> MACPISQSVSQPVDERLTRAAIFLVVTINPGKAAEVAVRTLCGTLSSLVRGVGFRILDGGLSCVMGVSSGGWERLFGDEKPEYLHVFQEINGVHHAPSTPGDLLFHIRAARMDLCFELASRILSDLGSSVCVVDSVQGFRYFDDRDLLGFVDGTENPVAQAAVDATLIGEEDHTFSGGSYVIVQKYLHDLDKWNAIPVEQQEKIIGREKLSDIELKDADKPSYAHNVLTSIEEDGEDVDILRDNMPFGDPGKGEFGTYFIGYSRKPARIERMLENMFVGNPPGNYDRILDVSRAITGTLFFIPTVSFLDSVEPQPSVSQQTDDAKYIYDSPGTKGESGSLNIGSLKKEVQDEENLYFQGGSGGHHHHHHH

Encapsulins are self-assembling protein nanocompartments capable of selectively encapsulating dedicated cargo proteins, including enzymes involved in iron storage, sulfur metabolism, and stress resistance. Encapsulation is mediated by specific cargo protein motifs known as targeting peptides (TPs), though the structural basis for encapsulation of the largest encapsulin cargo class, dye-decolorizing peroxidases (DyPs), is currently unknown. In this study, we report the structural and functional analysis of a DyP encapsulin system from a Gram-negative pathogen – Klebsiella pneumoniae (Kp). DyPs are ubiquitous, often homohexameric, heme-containing enzymes, named for their ability to oxidize and degrade a wide range of synthetic dyes – with concomitant reduction of hydrogen peroxide to water.

To investigate the influence of encapsulation on KpDyP and to compare the activities of encapsulated and free enzyme, a C-terminally His-tagged KpDyP construct (40.6 kDa) was heterologously expressed and purified. The structure of the free KpDyP hexamer was determined to 2.4 Å via D3 symmetry refinement followed by local refinement. The overall structure corroborates our biophysical and imaging analyses and confirms that free KpDyP exists as a catalytically competent hexamer. Cryo-EM density for a non-covalently bound heme cofactor – one per subunit – is clearly visible. The heme group is coordinated by residue His225, representing the proximal ligand to the heme iron. Arg242 is the residue closest to the heme iron on the distal face of the heme group. Moreover, the heme cofactor is substantially buried, with the entrance to the active site partially obstructed by an adjacent subunit at the two-fold interface. The KpDyP surface was found to be predominantly negatively charged, which is in agreement with its theoretical isoelectric point (pI) of 4.6552. The entrance to the active site is also highly negatively charged. In line with the predicted disordered state of the C-terminus, the last 60 residues – including the TP – are unresolved, which is generally observed for encapsulin cargo proteins in solution.>[2x]AVVKDFDISKFLGFW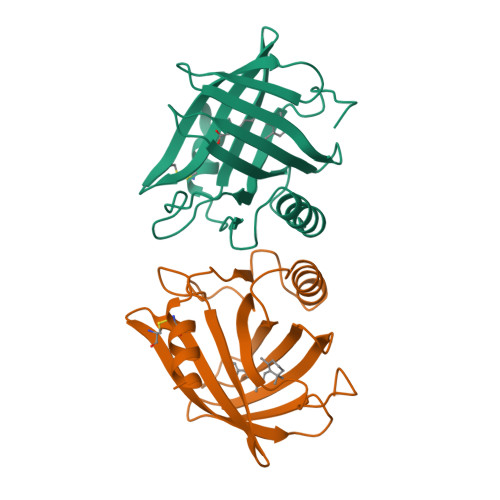YEIAFASKMGTPGLAHKEEKMGAMVVELKENLLALTTTYYSEDHCVLEKVTATEGDGPAKFQVTRLSGKKEVVVEATDYLTYAIIDITSLVAGAVHRTMKLYSRSLDDNGEALYNFRKITSDHGFSETDLYILKHDLTCVKVLQSAAES>[2x]MVLYFIGLGLYDERDITVKGLEIAKKCDYVFAEFYTSLMAGTTLGRIQKLIGKEIRVLSREDVELNFENIVLPLAKENDVAFLTPGDPLVATTHAELRIRAKRAGVESYVIHAPSIYSAVGITGLHIYKFGKSAMVAYPEGNWFPTSYYDVIKENAERGLHTLLFLDIKAEKRMYMTANEAMELLLKVEDMKKGGVFT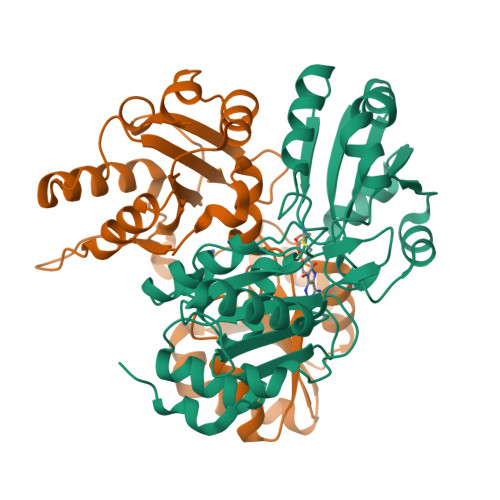DDTLVVVLARAGSLNPTIRAGYVKDLIREDFGDPPHILIVPGKLHIVEAEYLVEIAGAPREILRVNV> PTPVEVSQLTYNADTIGNWVPPTELKQTYTQDITGLKP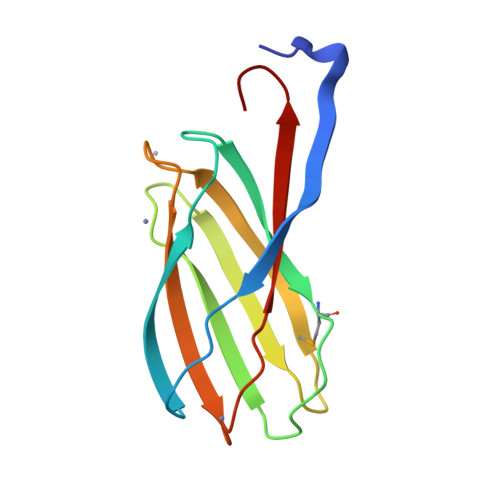NSKFIIVPYMDRVSSEVLQKCTITCNEVDAVGSISYFDTSAIKCDGYISFQANSIGEATFTLVTDYQGAVDPKPYQYRIIRAIVGNN> KPRIDMHSHFFPRISEQEAAKFDANHAPWLQVSAKGDTGSIMMGKNNFRPVYQALWDPAFRIEEMDAQGVDVQVTCATPVMFGYTWEANKAAQWAERMNDFALEFAAHNPQRIKVLAQVPLQDLDLACKEASRAVAAGHLGIQIGNHLGDKDLDDATLEAFLTHCANEDIPILVHPWDMMGGQRMKKWMLPWLVAMPAETQLAILSLILSGAFERIPKSLKICFGHGGGSFAFLLGAVD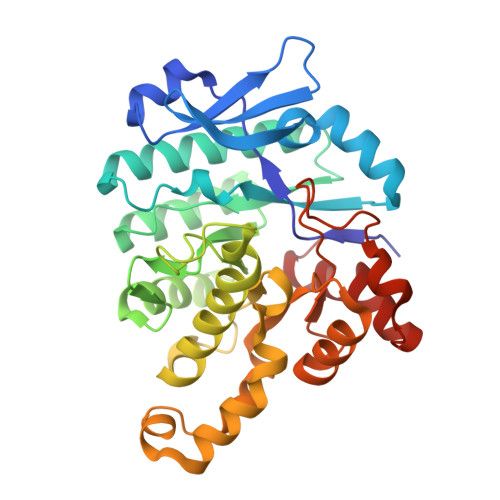NAWRHRDIVREDCPRPPSEYVDRFFVDSAVFNPGALELLVSVMGEDRVMLGSDYPFPLGEQKIGGLVLSSNLGESAKDKIISGNASKFFNIN>[3x]KPQIPKDKSKVAGYIEIPDADIKEPVYPGPATPEQLNRGVSFAEENESLDDQNISIAGHTFIDRPNYQFTNLKAAKKGSMVYFKVGNETRKYKMTSIRDVKPTDVGVL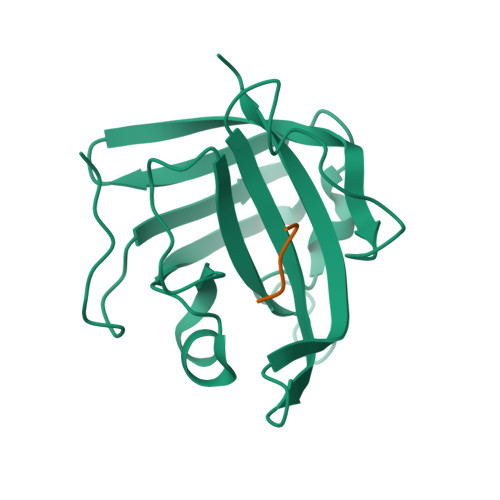DEQKGKDKQLTLITADDYNEKTGVWEKRKIFVATEVK;> LPETG>[2x]MKMYEVKEFSSGKRKLEDYKSII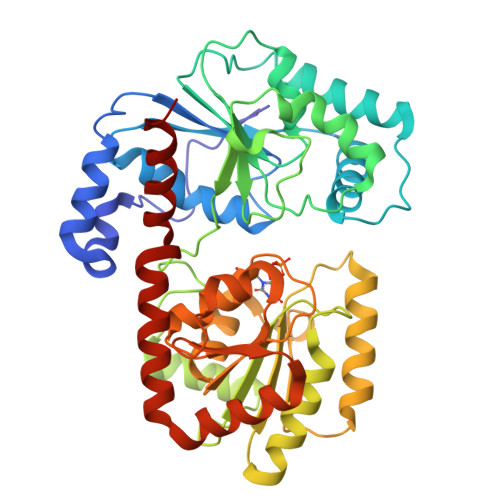GEEEVSKIQEKAEKLKGRSFVHVNSTSFGGGVAEILHSLVPLLRSIGIEARWFVIEGPTEFFNVTKTFHNALQGNESLKLTEEMKELYLNVNRENSKFIDLSSFDYVLVHDPQPAALIEFYEKKSPWLWRCHIDLSSPNREFWEFLRRFVEKYDRYIFHLPEYVQPELDRNKAVIMPPSIDPLSEKNVELKQTEILRILERFDVDPEKPIITQVSRFDPWKGIFDVIEIYRKVKEKIPGVQLLLVGVMAHDDPEGWIYFEKTLRKIGEDYDVKVLTNLIGVHAREVNAFQRASDVILQMSIRAGFGLTVTEAMWKGKPVIGRAVGGIKFQIVDGETGFLVRDANEAVEVVLYLLKHPEVSKEMGAKAKERVRKNFIITKHMERYLDILNSLGG>MTATASDDEAVTALALSAAKGNGRALEAFIKATQQDVWRFVAYLSDVGSADDLTQETFLRAIGAIPRFS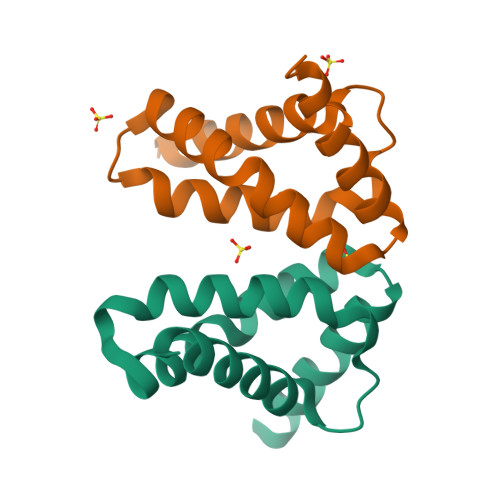ARSSARTWLLAIARHVVADHIRHVRSRPRTTRGARPEHLIDGD[2x]> QCK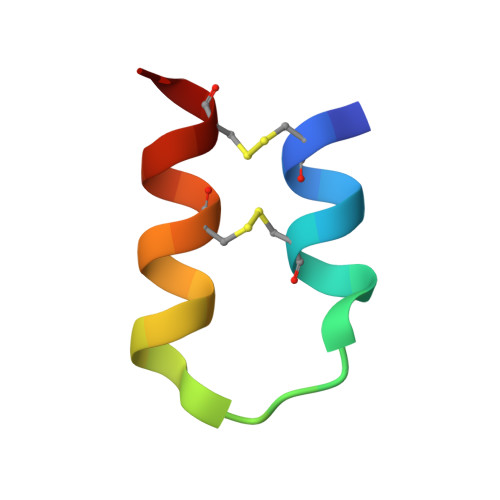VMCYAQRHSSPELLRRCLDNCEK> MDVDEMLKQVEILRRLGAKRIAVRSDDWRILQEALKKGGDILIVDATDVDEMLKQVEILRRLGAKEIAVRSDDWRILQEALKKGGDILIVDATDVDEMLKQVEILRRLGAKRIAVRSDDWRILQEALKKGGDILIVDATDVDEMLKQVEILRRLGAKEIAVRSDDWRILQEALKK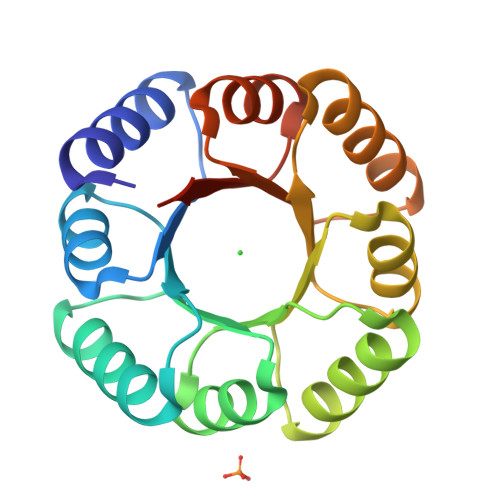GGDILIVDATLEHHHHHH> MFEARLVQGSILKKVLEALKDLINEACWDISSSGVNLQSMDSSHVSLVQLTLRSEGFDTYRCDRNLAMGVNLTSMSKILKCAGNEDIITLRAEDNADTLALVFEAPNQEKVSDYEMKLMDLDVEQLGIPEQEYSCVVKMPSGEFARICRDLSHIG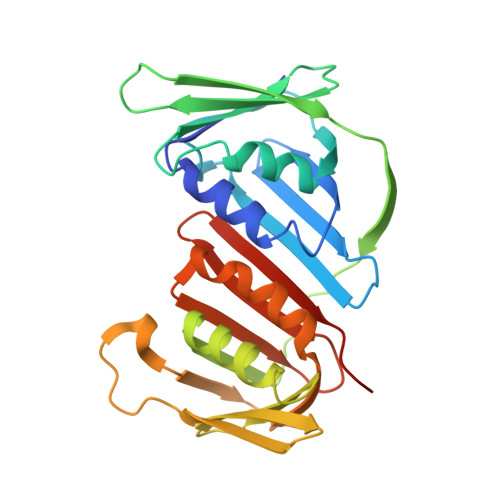DAVVISCAKDGVKFSASGELGNGNIKLSQTSNVDKEEEAVTIEMNEPVQLTFALRYLNFFTKATPLSSTVTLIMSADVPLVVEYKIADMGHLKYYLAPKIEDEEGS> PELPEVETVRRELEKRIVGQKIISIEATYPRMVLTGFEQLKKELTGKTIQGISRRGKYLIFEIGDDFRLISHLRMEGKYRLATLDAPREKHDHLTMKFADGQLIYADVRKFGTWELISTDQVLPYFLKKKIGPEPTYEDFDEKLFREKLRKSTKKIKPYLLEQTLVAGLGNIYVDEVLWLAKIHPEKETNQLIESSIHLLHDSIIEILQKAIKLGGSS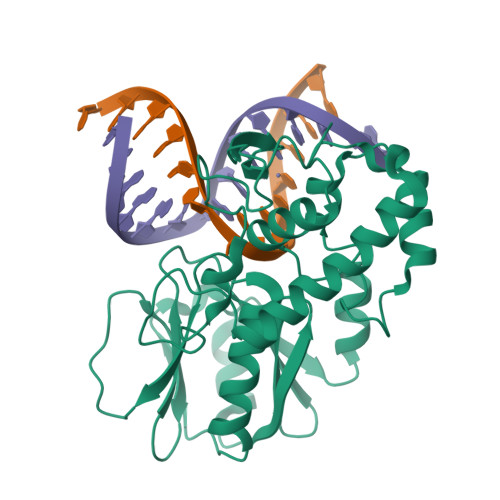IRTYSALGSTGKMQNELQVYGKTGEKCSRGHGAEIQKIKVAGRGTHFCPVCQQK Here, a series of new methods are presented based on the use of a low X-ray-background film as a crystallization support and a photoablation laser that enable the automation of major operations required for the preparation of crystals for X-ray diffraction experiments. In this approach, the controlled removal of the mother liquor before crystal mounting simplifies the cryocooling process, in many cases eliminating the use of cryoprotectant agents, while crystal-soaking experiments are performed through diffusion, precluding the need for repeated sample-recovery and transfer operations. We have previously shown that the transfer of crystals to X-ray data-collection pins can be automated through the so-called CrystalDirect approach, which relies on the use of a thin, low X-ray-background film as a crystallization support from which crystals are recovered by excising the film with a laser beam and attaching it to an X-ray data-collection pin. The CrystalDirect system enables the automation of sample mounting and cryocooling and can contribute to closing the automation gap that currently exists between crystallization and X-ray data collection.

Some of these crystals grew in conditions that require the addition of cryoprotectants when processed by standard manual methods. However, in all cases tested the automated laser mounting and direct cryocooling after liquid removal with the CrystalDirect robot produced samples with very good diffraction properties leading to high-quality structural models.

> GHRTLASTPALWASIPCPRSELRLDLVLPSGQSFRWREQSPAHWSGVLADQVWTLTQTEEQLHCTVYRGDKSQASRPTPDELEAVRKYFQLDVTLAQLYHHWGSVDSHFQEVAQKFQGVRLLRQDPIECLFSFICSSNNNIARITGMVERLCQAFGPRLIQLDDVTYHGFPSLQALAGPEVEAHLRKLGLGYRARYVSASARAILEEQGGLAWLQQLRESSYEEAHKALCILPGVGTKVADCICLMALDKPQAVPVDVHMWHIAQRDYSWHPTTSQAKGPSPQTNKELGNFFRSLWGPYAGWAQAVLFSADL(2S)-2-hydroxy-3-(morpholin-4-yl)propane-1-sulfonic acid | C7 H15 N O5 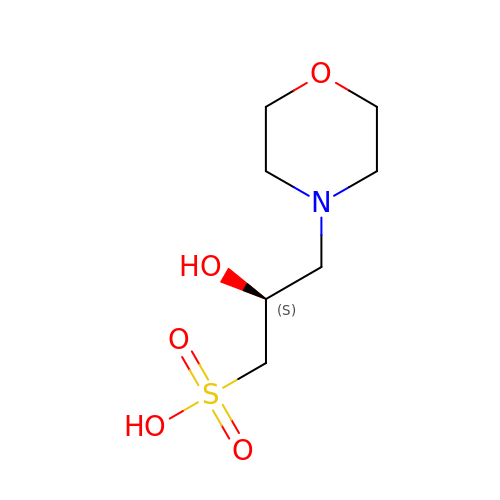S | NUFBIAUZAMHTSP-ZETCQYMHSA-N>EDKYTDKYDNINLDEILANKRLLVAYVNCVMERGKCSPEGKELKEHLQDAIENGCKKCTENQEKGAYR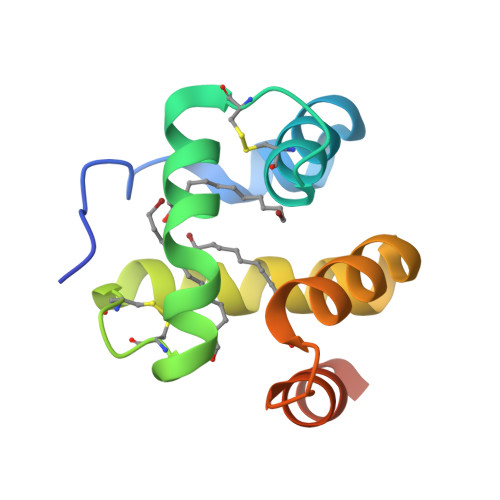VIEHLIKNEIEIWRELTAKYDPTGNWRKKYEDRAKAAGIVIPEE[2x]>FQGVIKIRYPDDGQWPEAPIDGDGDGNPEFYIEINPWNIQSAEGYAEMTYNLSTGVLHYVQALDDITLKNGGSWVHGYPEIFYGNKPWNNNYATDGEVPLPGKVSNLSNFY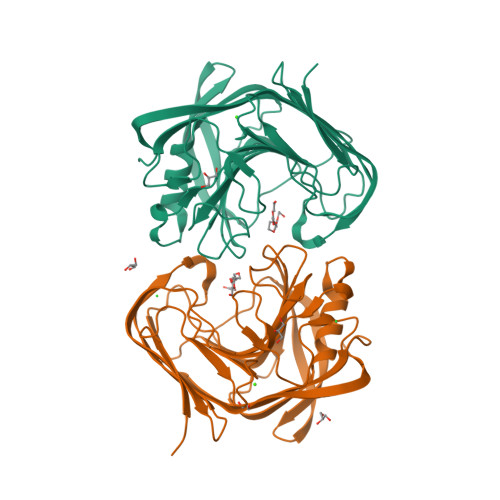LSVSYKLLPKNGLPINFAIESWLTREPWRNSGINSDEQELMIWLYYDGLQPAGSKVKEIIVPIVVNGTPVNATFEVWKANIGWEYIAFRIKTPIKEGTVTIPYGAFISAAANVTSLANYTELYLEDVEVGTEYGTPSTTSAHLEWWFYNVSLEYRPGEPLLSQPPAEGSAP[2x]>MSNEVSIKELIEKAKVAQKKLEAYSQEQVDVLVKALGKVVYDNAEMFAKEAVEETEMGVYEDKVAKCHLKSGAIWNHIKDKKTVGIIKEEPERALVYVAKPKGVVAATTPITNPVVTPMCNAMAAIKGRNTIIVAPHPKAKKVSAHTVELMNAELKKLGAPENIIQIVEAPSREAAKELMESADVVIATGGAGRVKAAYSSGRPAYGVGPGNSQVIVDKGYDYNKAAQDIITGRKYDNGIICSSEQSVIAPAEDYDKVIAAFVENGAFYVEDEETVEKFRSTLFKDGKINSKIIGKSVQIIADLAGVKVPEGTKVIVLKGKGAGEKDVLCKEKMCPV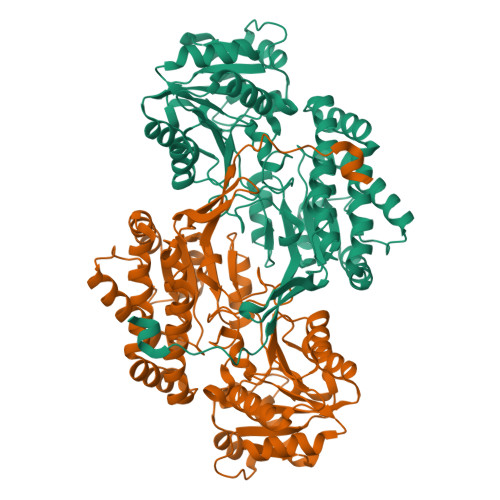LVALKYDTFEEAVEIAMANYMYEGAGHTAGIHSDNDENIRYAGTVLPISRLVVNQPATTAGGSFNNGFNPTTTLGCGSWGRNSISENLTYEHLINVSRIGYFNKEAKVPSYEEIWG[4x]(2S,3AS,7AS)-1-[(2S)-2-{[(2S)-2-CYCLOHEXYL-2-({[(2R)-4-NITRO-2H-PYRROL-2-YL]CARBONYL}AMINO)ACETYL]AMINO}-3,3-DIMETHYLBUTANOYL]-N-{(1S)-1-[(1R)-2-(CYCLOPROPYLAMINO)-1-HYDROXY-2-OXOETHYL]BUTYL}OCTAHYDRO-1H-INDOLE-2-CARBOXAMIDE 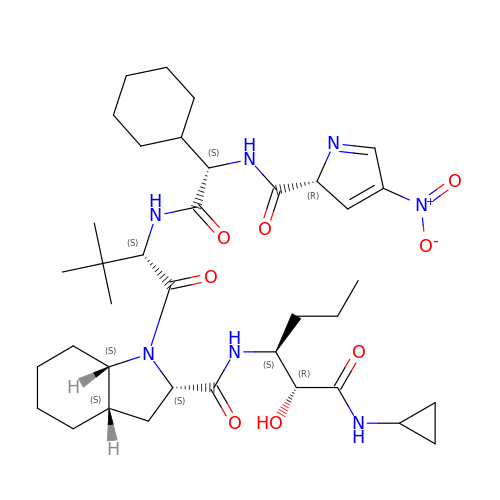| C37 H57 N7 O8 | HXPWPXJRIXYIRJ-MGNUMPGCSA-N>[2x]MNGEAICSALPTIPYHKLADLRYLSRGASGTVSSARHADWRVQVAVKHLHIHTPLLDSERKDVLREAEILHKARFSYILPILGICNEPEFLGIVTEYMPNGSLNELLHRKTEYPDVAWPLRFRILHEIALGVNYLHNMTPPLLHHDLKTQNILLDNEFHVKIADFGLSKWRMMSLSQSRSS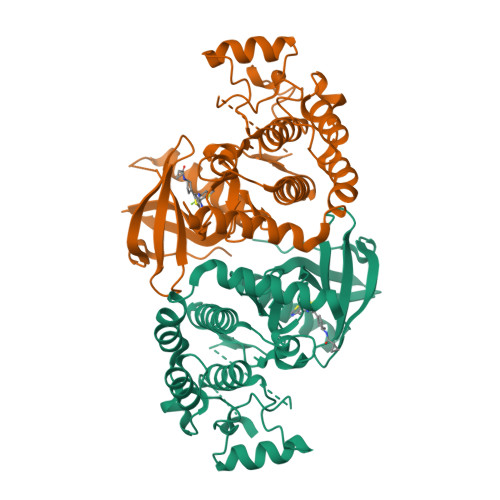KSAPEGGTIIYMPPENYEPGQKSRASIKHDIYSYAVITWEVLSRKQPFEDVTNPLQIMYSVSQGHRPVINEESLPYDIPHRARMISLIESGWAQNPDERPSFLKCLIELEPVLRTFEEITFLEAVIQLKKTKLQS> ATANLHLYQDLQREVGSLKEINFMLSVLQKEFLHLSKEFATTSKDLSAVSQDFYSCLQGFRDNYKGFES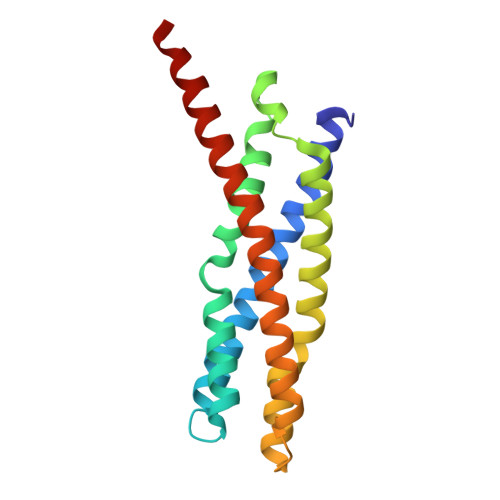LLDEYKNSTEEMRKLFSQEIIADLKGSVASLREEIRFLTPLAEEVRRLAHNQQSLTAAIEELKTIRDSLRDEIGQLSQLSKTLTSQIALQRKLEHHHHHH>[2x]CPRFLKVKNWETEVVLTDTLHLKSTLETGCTEYICMGSIMHPSQHARRPEDVATKDQLFPLAKEFIDQYYSSIKRFGSKAHMERLEEVNKEIDTTSTYQLKDTELIYGAKHAWRNASRCVGRIQWSKLQVFDARDCTTAHGMFNYICNHVKYATNKGNLRSAITIFPQRTDGKHDFRVWNSQLIRYAGYKQPDGSTLGDPANVQFTEICIQQGWKPPRGRFDVLPLLL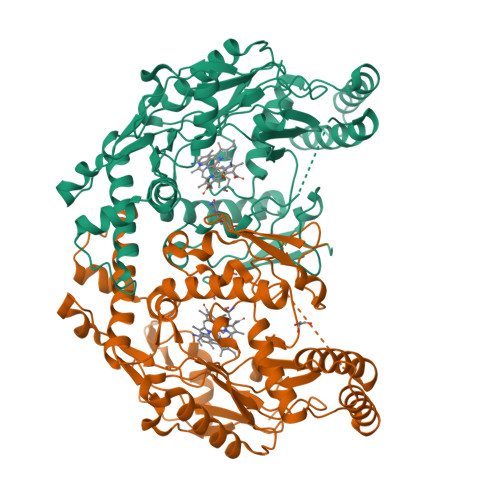QANGNDPELFQIPPELVLEVPIRHPKFEWFKDLGLKWYGLPAVSNMLLEIGGLEFSACPFSGWYMGTEIGVRDYCDNSRYNILEEVAKKMNLDMRKTSSLWKDQALVEINIAVLYSFQSDKVTIVDHHSATESFIKHMENEYRCRGGCPADWVWIVPPMSGSITPVFHQEMLNYRLTPSFEYQPDPWNTHVWK>[14x]GQAFRKFLPLFDRVLVERSAAETVTKGGIMLPEKSQGKVLQATVVAVGSGSKGKGGEIQPVSVKVGDKVLLPEYGGTKVVLDDKDYFLFRDGDILGKYVD;>GSAKDVKFGADARALMLQGVDLLADAVAVTMGPKGRTVIIEQSWGSPKVTKDGVTVAKSIDLKDKYKNIGAKLVQDVANNTNEEAGDGTTTATVLARSIAKEGFEKISKGANPVEIRRGVMLAVDAVIAELKKQSKPVTTPEEIAQVATISAN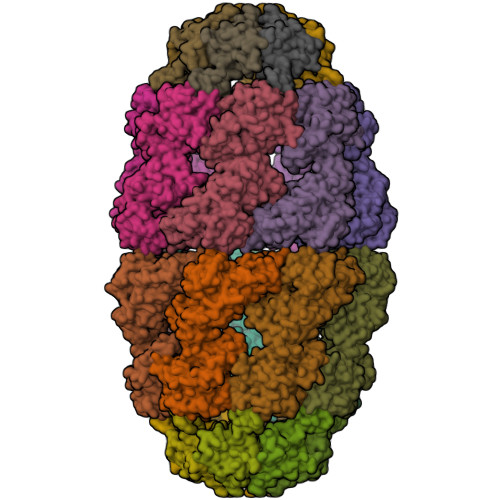GDKEIGNIISDAMKKVGRKGVITVKDGKTLNDELEIIEGMKFDRGYISPYFINTSKGQKCEFQDAYVLLSEKKISSIQSIVPALEIANAHRKPLVIIAEDVDGEALSTLVLNRLKVGLQVVAVKAPGFGDNRKNQLKDMAIATGGAVFGEEGLTLNLEDVQPHDLGKVGEVIVTKDDAMLLKGKGDKAQIEKRIQEIIEQLDVTTSEYEKEKLNERLAKLSDGVAVLKVGGTSDVEVNEKKDRVTDALNATRAAVEEGIVLGGGCALLRCIPALDSLTPANEDQKIGIEIIKRTLKIPAMTIAKNAGVEGSLIVEKIMQSSSEVGYDAMAGDFVNMVEKGIIDPTKVVRTALLDAAGVASLLTTAEVVVTEIPKE[14x]>[2x]KFGWIKGVLVRCMLNIWGVMLFIRMTWIVGQAGIAYSCIIVIMATVVTTITGCSTSAIATNGFVRGGGAYYLISRSLGPEFGGSIGLIFA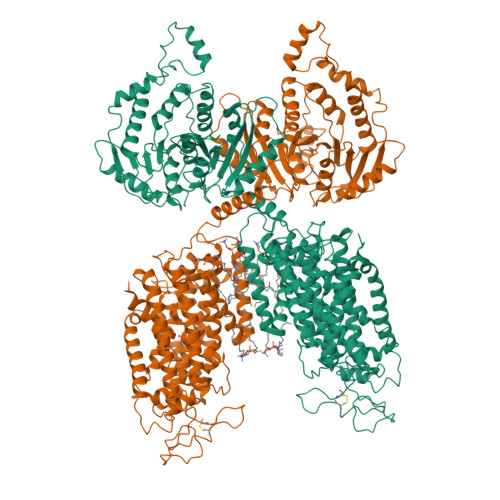FANAVAVAMYVVGFAETVVELLMDSGLLMIDQTNDIRVIGTITVILLLGISVAGMEWEAKAQIFLLVILITAIFNYFIGSFIAVDSKKKFGFFSYDAGILAENFGPDFRGQTFFSVFSIFFPAATGILAGANISGDLADPQMAIPKGTLLAILITGLVYVGVAISAGACIVRDATGIESNFTLISNCTDAACKYGYDFSSCRPTVEGEVSSCKFGLHNDFQVMSVVSGFSPLISAGIFSATLSSALASLVSAPKVFQALCKDNIYPGIAIFGKGYGKNNEPLRGYFLTFGIALAFILIAELNVIAPIISNFFLASYALINFSVFHASLANSPGWRPSFKYYNMWASLAGAILCCVVMFIINWWAALLTNVIVLSLYIYVSYKKPDVNWGSSTQALTYHQALTHSLQLCGVADHIKTFRPQCLVMTGAPNSRPAILHLVHAFTKNVGLMLCGHVRISSRRPNFKELNSDMLRYQRWLLNNNSKAFYTCVVAEDLRQGTQYMLQAAGLGRLRPNTLVIGFKNDWRIGDIKEVETYINLIHDAFDFQYGVVILRLREGLDISHIQGQDDSSGMKDVVVSVDISKDSDGDSSKPSSKATSVQNSPAVQKDKKSPTVPLNVADQRLLDSQQFQQKQGKGTVDVWWLFDDGGLTLLIPYLIANKKKWKDCKIRVFIGGKINRIDHDRRAMATLLSKFRIDFSDITVLGDINTKPKSEGLTEFAEMIEPYKLREDDMEQEAAEKLKSEEPWRITDNELELYKAKGNRQIRLNELLKEHSSTANLIVMSMPLARKGAVSSALYMAWLDTLSKDLPPILLVRGNHQSVLTFYS> MKDLLKFLKAQTKTEEFDAIKIALASPDMIRSWSFGEVKKPETINYRTFKPERDGLFCARIFGPVKDYECLCGKYKRLKHRGVICEKCGVEVTQTKVRRERMGHIELASPTAHIWFLKSLPSRIGLLLDMPLRDIERVLYFESYVVIEGGMTNLERQQILTEEQYLDALEEFGDEFDAKMGAEAIQALLKSMDLEQECEQLREELNETNSETKRKKLTKRIKLLEAFVQSGNKPEWMILTVLPVLPPDLRPLVPLDGGRFATSDLNDLYRRVINRNNRLKRLLDLAAPDIIVRNEKRMLQEAVDALLDNGRRGRAITGSNKRPLKSLADMIKGKQGRFRQNLLGKRVDYSGRSVITVGPYLRLHQCGLPKKMALELFKPFIYGKLELRGLATTIKAAKKMVEREEAVVWDILDEVIREHPVLLNRAPTLHRLGIQAFEPVLIEGKAIQLHPLVCAAYNADFDGDQMAVHVPLTLEAQLEARALMMSTNNILSPANGEPIIVPSQDVVLGLYYMTRDCVNAKGEGMVLTGPKEAERLYRSGLASLHARVKVRITEYEKDANGELVAKTSLKDTTVGRAILWMIVPKGLPYSIVNQALGKKAISKMLNTCYRILGLKPTVIFADQIMYTGFAYAARSGASVGIDDMVIPEKKHEIISEAEAEVAEIQEQFQSGLVTAGERYNKVIDIWAAANDRVSKAMMDNLQTETVINRDGQEEKQVSFNSIYMMADSGARGSAAQIRQLAGMRGLMAKPDGSIIETPITANFREGLNVLQYFISTHGARKGLADTALKTANSGYLTRRLVDVAQDLVVTEDDCGTHEGIMMTPVIEGGDVKEPLRDRVLGRVTAEDVLKPGTADILVPRNTLLHEQWCDLLEENSVDAVKVRSVVSCDTDFGVCAHCYGRDLARGHIINKGEAIGVIAAQSIGEPGTQLTMRTFHIGGAASRAAAESSIQVKNKGSIKLSNVKSVVNSSGKLVITSRNTELKLIDEFGRTKESYKVPYGAVLAKGDGEQVAGGETVANWDPHTMPVITEVSGFVRFTDMIDGQTITRQTDELTG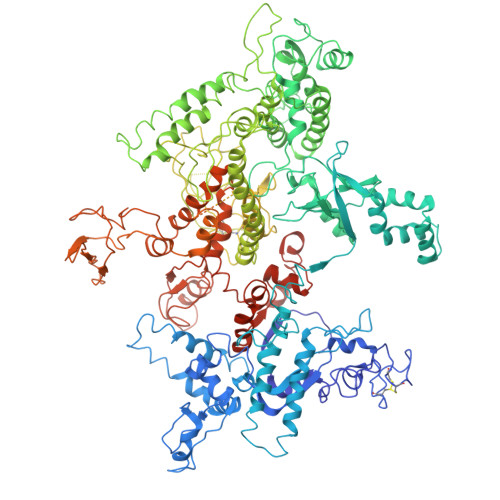LSSLVVLDSAERTAGGKDLRPALKIVDAQGNDVLIPGTDMPAQYFLPGKAIVQLEDGVQISSGDTLARIPQESGGTKDITGGLPRVADLFEARRPKEPAILAEISGIVSFGKETKGKRRLVITPVDGSDPYEEMIPKWRQLNVFEGERVERGDVISDGPEAPHDILRLRGVHAVTRYIVNEVQDVYRLQGVKINDKHIEVIVRQMLRKATIVNAGSSDFLEGEQVEYSRVKIANRELEANGKVGATYSRDLLGITKASLATESFISAASFQETTRVLTEAAVAGKRDELRGLKENVIVGRLIPAGTGYAYHQDRMRRRAAGEAPAAPQVTAEDASASLAELLNAGLGGSDNELEVHHHHHH>[2x]MRGGALHQNRRVTLPSVPLPAVLPPLTDHAGAVAHLS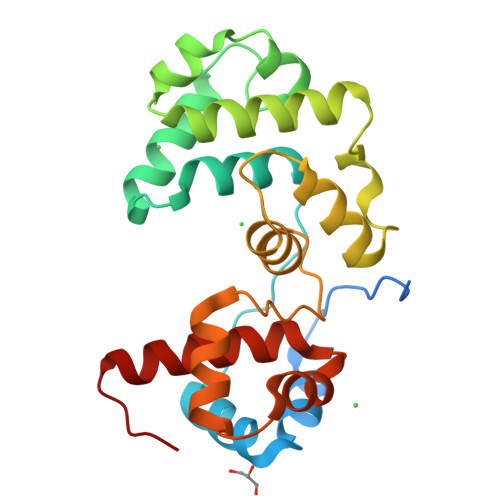RDPVLAQVTSLCGELPVLAPTPDPFGRLVRSVAGQQLSVKAAQAIYGRLEGLPGGVVPAALLKVSGDDLRGVGLSWAKVRTVQAAAAAAVSGQIDFAHLSGQPDELVIAELVQLPGIGRWTAEMFLLFALARPDVFSSGDLALRQGVERLYPGEDWRDVTARWAPYRSLASRYLWANSARMQAGGAPL5'-deoxy-5'-({[(2R)-2-{[2-({N-[(2R)-2-hydroxy-3,3-dimethyl-4-(phosphonooxy)butanoyl]-beta-alanyl}amino)ethyl]sulfanyl}-2-(3-hydroxyphenyl)ethyl]sulfonyl}amino)adenosine | 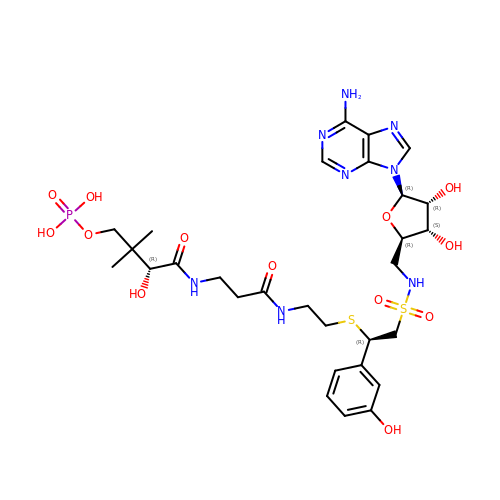C29 H43 N8 O13 P S2 | ADMPPCCGBBJHMD-XCYBABBZSA-N>GSFTEELHLIPPLNFSMVDNGIFRSGFPDSANFSFLQTLGLRSIIYLCPEPYPESNLQFLKSNGIRLFQFGIEGNKEPFVNIPDHKIRMALKVLLDEKNHPVLIHSKRGKHRTGCLVGCLRKLQKWCLTSIFDEYQRFAAAKARVSDQRFMEIFDVSSFSHIPMSFSCSIR[2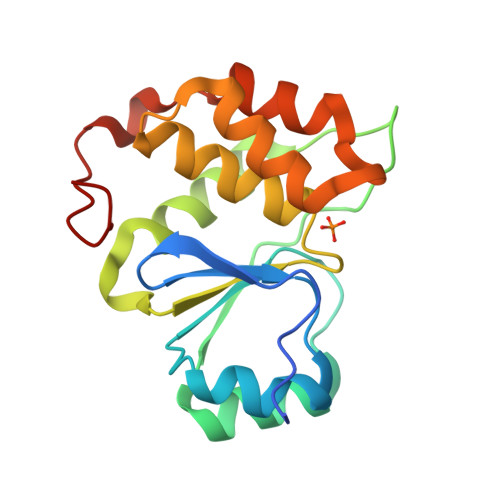x]> SATRRYYLGAVELSWDYMQSDLGELPVDARFPPRVPKSFPFNTSVVYKKTLFVEFTDHLFNIAKPRPPWMGLLGPTIQAEVYDTVVITLKNMASHPVSLHAVGVSYWKASEGAEYDDQTSQREKEDDKVFPGGSHTYVWQVLKENGPMASDPLCLTYSYLSHVDLVKDLNSGLIGALLVCREGSLAKEKTQTLHKFILLFAVFDEGKSWHSETKNSLMQDRDAASARAWPKMHTVNGYVNRSLPGLIGCHRKSVYWHVIGMGTTPEVHSIFLEGHTFLVRNHRQASLEISPITFLTAQTLLMDLGQFLLFCHISSHQHDGMEAYVKVDSCPEEPQLRMKNNEEAEDYDDDLTDSEMDVVRFDDDNSPSFIQIRSVAKKHPKTWVHYIAAEEEDWDYAPLVLAPDDRSYKSQYLNNGPQRIGRKYKKVRFMAYTDETFKTREAIQHESGILGPLLYGEVGDTLLIIFKNQASRPYNIYPHGITDVRPLYSRRLPKGVKHLKDFPILPGEIFKYKWTVTVEDGPTKSDPRCLTRYYSSFVNMERDLASGLIGPLLICYKESVDQRGNQIMSDKRNVILFSVFDENRSWYLTENIQRFLPNPAGVQLEDPEFQASNIMHSINGYVFDSLQLSVCLHEVAYWYILSIGAQTDFLSVFFSGYTFKHKMVYEDTLTLFPFSGETVFMSMENPGLWILGCHNSDFRNRGMTALLKVSSCDKNTGDYYEDSYEDISAYLLSKNNAIEPRSDPLAWDNHYGTQIPKEEWKSQEKSPEKTAFKKKDTILSLNACESNHAIAAINEGQNKPEIEVTWAKQGRTERLCSQNPPVLKRHQREITRTTLQSDQEEIDYDDTISVEMKKEDFDIYDEDENQSPRSFQKKTRHYFIAAVERLWDYGMSSSPHVLRNRAQSGSVPQFKKVVFQEFTDGSFTQPLYRGELNEHLGLLGPYIRAEVEDNIMVTFRNQASRPYSFYSSLISYEEDQRQGAEPRKNFVKPNETKTYFWKVQHHMAPTKDEFDCKAWAYFSDVDLEKDVHSGLIGPLLVCHTNTLNPAHGRQVTVQEFALFFTIFDETKSWYFTENMERNCRAPCNIQMEDPTFKENYRFHAINGYIMDTLPGLVMAQDQRIRWYLLSMGSNENIHSIHFSG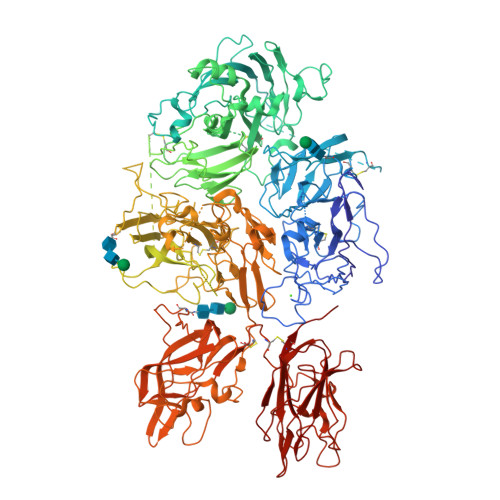HVFTVRKKEEYKMALYNLYPGVFETVEMLPSKAGIWRVECLIGEHLHAGMSTLFLVYSNKCQTPLGMASGHIRDFQITASGQYGQWAPKLARLHYSGSINAWSTKEPFSWIKVDLLAPMIIHGIKTQGARQKFSSLYISQFIIMYSLDGKKWQTYRGNSTGTLMVFFGNVDSSGIKHNIFNPPIIARYIRLHPTHYSIRSTLRMELMGCDLNSCSMPLGMESKAISDAQITASSYFTNMFATWSPSKARLHLQGRSNAWRPQVNNPKEWLQVDFQKTMKVTGVTTQGVKSLLTSMYVKEFLISSSQDGHQWTLFFQNGKVKVFQGNQDSFTPVVNSLDPPLLTRYLRIHPQSWVHQIALRMEVLGCEAQDLY> MGHHHHHHHHHHSSGHIEGRHMFSKNAVKLHATPPSVAAPPTGAPEVAAERLEPRVEEKDGYWILKEQFRKGINPQEKVKIEKEPMKLFMENGIEELAKIPIEEIDQSKLTKDDIDVRLKWLGLFHRRKNQYGRFMMRLKLPNGVTTSAQTRYLASVIRKYGKEGCADITTRQNWQIRGVVLPDVPEILKGLAEVGLTSLQSGMDNVRNPVGNPLAGIDPEEIVDTRPYTNLLSQFITGNSRGNPAVSNLPRKWNPCVVGSHDLYEHPHINDLAYMPATKDGRFGFNLLVGGFFSAKRCDEAIPLDAWVPADDVVPVCRAILEAFRDLGFRGNRQKCRMMWLIDELGVEGFRAEVEKRM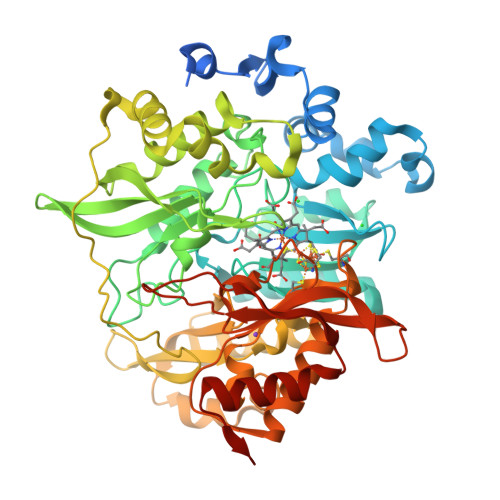PQQQLERASPEDLVQKQWERRDYLGVHPQKQEGYSFIGLHIPVGRVQADDMDELARLADEYGSGEIRLTVEQNIIIPNIETSKIEALLKEPVLSTFSPDPPILMKGLVACTGNQFCGQAIIETKARSLKITEEVQRQVSLTKPVRMHWTGCPNTCAQVQVADIGFMGCLTRDKNGKTVEGADVFLGGRIGSDSHLGEVYKKAVPCDDLVPLVVDLLVNNFGAVPREREETED>MLGLKTSIIGRRVIYFQEITSTNEFAKTSYLEEGTVIVADKQTMGHGRLNRKWESPEGGLWLSIVLSPKVPQKDLPKIVFLGAVGVVETLKEFSIDGRIKWPNDVLVNYKAIAGVLVEGKGDKIVLGIGLNVNNKVPNGATSMKLELGSEVPLLSVFRSLITNLDRLYLNFLKNPMDILNLVRDNMILGVRVKILGDGSFEGIAEDIDDFGRLIIRLDSGEVKKVIYGDVSLRFL[2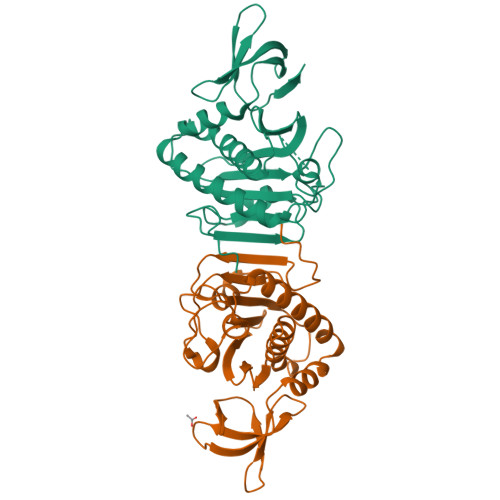x]>[2x]GSMSSDAQWLTAEERDQLIPGLKAAGWSELSERDAIYKEFSFKNFN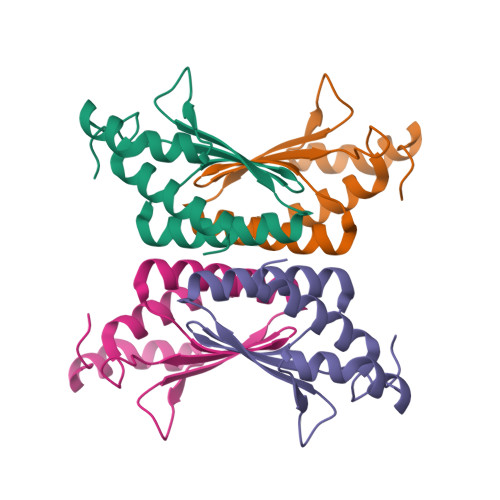QAFGFMTRVALQAEKMNHHPEWFNVYNKVQITLTSHDCGGLTKRDVKLAQFIEKAAASL>[20x]MAEASIEKTQILQKYLELDQRGRIIAEYVWIDGTGNLRSKGRTLKKRITSIDQLPEWNFDGSSTNQAPGHDSDIYLKPVAYYPDPFRRGDNIVVLAACYNNDGTPNKFNHRHEAAKLFAAHKDEEIWFGLEQEYTLFDMYDDVYGWPKGGYPAPQGPYYCGVGAGKVYARDMIEAHYRACLY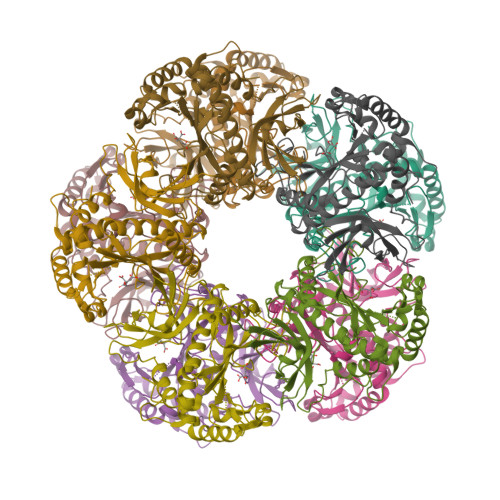AGLEISGINAEVMPSQWEFQVGPCTGIDMGDQLWMARYFLHRVAEEFGIKISFHPKPLKGDWNGAGCHANVSTKEMRQPGGTKYIEQAIEKLSKRHAEHIKLYGSDNDMRLTGRHETASMTAFSSGVANRGSSIRIPRSVAKEGYGYFEDRRPASNIDPYLVTGIMCETVCGAIDNADMTKEFERESS>[19x]TSIYPKFRAAAVQAAPIYLNLEASVEKSCELIDEAASNGAKLVAFPEAFLPGYPWFAFIGHPEYTRKFYHELYKNAVEIPSLAIQKISEAAKRNETYVCISCSEKDGGSLYLAQLWFNPNGDLIGKHRKMRASVAERLIWGDGSGSMMPVFQTRIGNLGGLMCWEHQVPLDLMAMNAQNEQVHVASWPGYFDDEISSR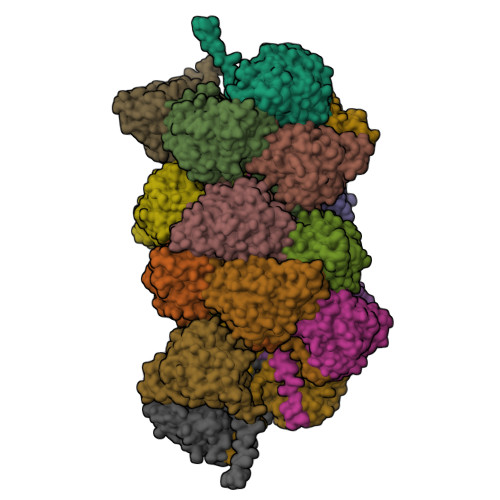YYAIATQTFVLMTSSIYTEEMKEMICLTQEQRDYFETFKSGHTCIYGPDGEPISDMVPAETEGIAYAEIDVERVIDYKYYIDPAGHYSNQSLSMNFNQQPTPVVKHLNHQKNEVFTYEDIQ> MKIYIQPLSVNSHTVEVLANSLPKIFNAEVFVLPASDVSLKCYNASRRQYNSTC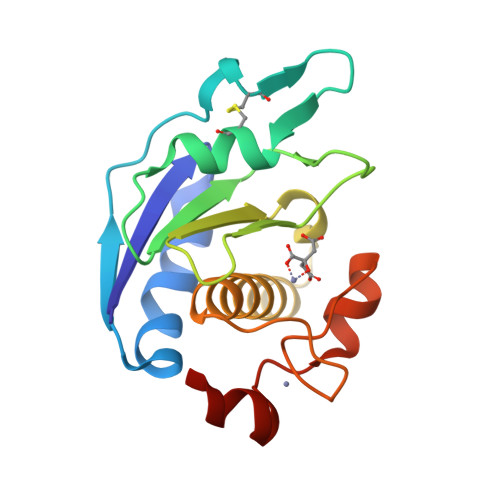ILRMLPPIKVTLGVTGKDIYAKGMNFVFGEAELGGARAVLSVFRLTTADSELYRERVVKEAVHEIGHVLGLKHCSNNCVMRFSNSVQDVDRKPVSFCRECASKIRY>[6x]MHLPNGAQIFVETSRGVEVEATAITNAENPVATVASKGDLAKGDYVIVTQSTWAKMVSRVLIVTDAQETSITLAGIDTSDTLVFPAGGTMSFAKIT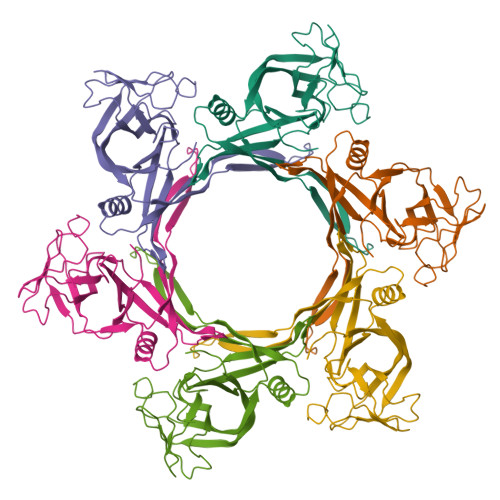GWTEIPCVQEIGQDGGEQQYYTYQCLSDDKEQQIPTFKSAVSLTYTFAHEFDNPIYPILRKLDSSGQVTAVRMYVPKASEMRMWAGILSFNDIPSTQVNEMETVELAVSLKGDFTFISSTLASPGA> AGAGADRTAATPAAANPAATEPVKWECPAGYEVKEGLNVDFPHKGMKRAFIVYPAKNVSGPAPVWVPMTGSVESTNDNLTVARSGANSILADHGYTVIAPVRA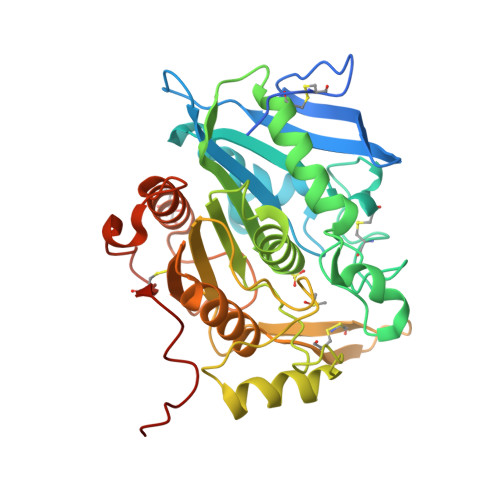CANQDPNIRGERCNGPGSNGWNWNPWFEGRAADPSGEHWKNDEGPDSSFFVAMVQCVGTKYKLDARRLFLGGICSGGTMTNRALLFRSNFWAGGLPISGEWYVTSDDGTPLSFDDARAAVAAAPTKIHQGRVGPYPLPAKVGPLIVMTVWGGEKDLWNCTRPDGSRFLCADYRPSTQAGSNFFSAQPDVVHVACSSTHGHMWPQLNTQEFNRWALDTLASHPKGSDPRSFKLTQPPEGYTCHVGPFTGLYASAWSHPQFEK>MDHLPIFCQLRDRDCLIVGGGDVAERKARLLLEAGARLTVNALTFIPQFTVWANEGMLTLVEGPFDETLLDSCWLAIAATDDDTVNQRVSDAAESRRIFCNVVDAPKAASFIMPSIIDRSPLMVAVSAGGTSPVLARLLREKLESLLPQHLGQVARYAGQLRARVKKQFATMGERRRFWEKFFVNDRLAQSLANADEKAVNATTERLFSEPLDHRGEVVLVGAGPGDAGLLTLKGLQQIQQADIVVYDRLVSDDIMNLVRRDADRVFVGKRAGYHCVPQEEI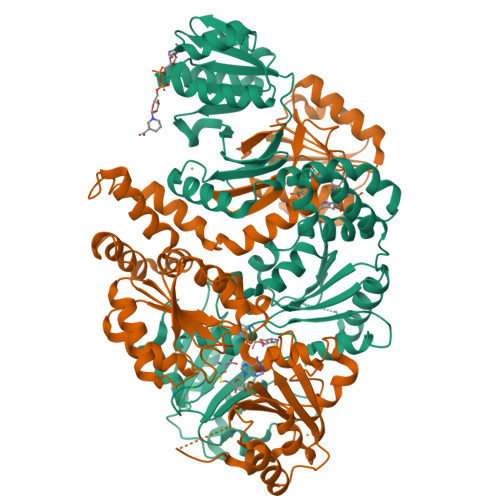NQILLREAQKGKRVVRLKGGDPFIFGRGGEELETLCHAGIPFSVVPGITAASGCSAYSGIPLTHRDYAQSVRLVTGHLKTGGELDWENLAAEKQTLVFYMGLNQAATIQEKLIAFGMQADMPVALVENGTSVKQRVVHGVLTQLGELAQQVESPALIIVGRVVALRDKLNWFSNH[2x]2-phenyl-N-(propan-2-yl)-6-[(thiophen-2-yl)sulfonyl]-4,5,6,7-tetrahydro-1H-pyrrolo[2,3-c]pyridine-1-carboxamide 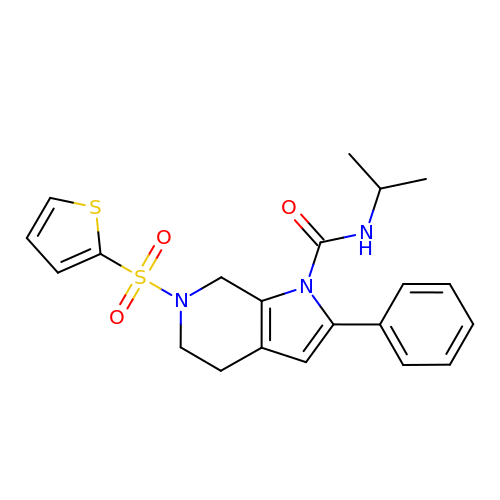| C21 H23 N3 O3 S2 | TYBYSTDSEWDDKH-UHFFFAOYSA-N> MIAQEPAALRPALGRLQQVALIVGGVAMLLAVAGAFLGAAQFFHSYIFAYFFWMALSLGGLLVLMINHLTQGVWGLMLRRLLEAAALTLPLMAILFLPIAAETLMGTHYLFPWTNPEVVANDEVVALKTPYLNVPFFLARAVIYFVLFIGMAYLLRQWSLEEDAKGFSDDLRGRFQRLSGP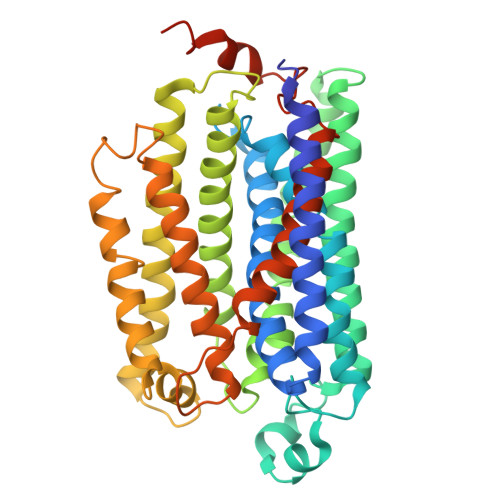GIVVLVMAWTFAATDWGMSLEPEWFSSMYPVTYIASMLILTFGGGIIALAVLKSRNLLPFGIPVDRLHDLGKFLFAFVAVWAYVNFSEYLIIWSGNVPELTPWHGHRSAGGWEILGIVMIFGHFLLPFMLLLSRFAKRRLANLTAIAIYLYLIEIVWYFWKIMPAFHPDGFHIHWLDLVTLIAIGGLWLGVFAWNLQRAPLLAPNDYRVPLLRRQEASGHGHGHHGKATAEHH>[4x]GPGNEVTLLDSRSVQGELGWIASPLEGGWEEVSIMDEKNTPIRTYQVCNVMEPSQNNWLRTDWITREGAQRVYIEIKFTLRDCNSLPGVMGTCKETFNLYYYESDNDKERFIRENQFVKID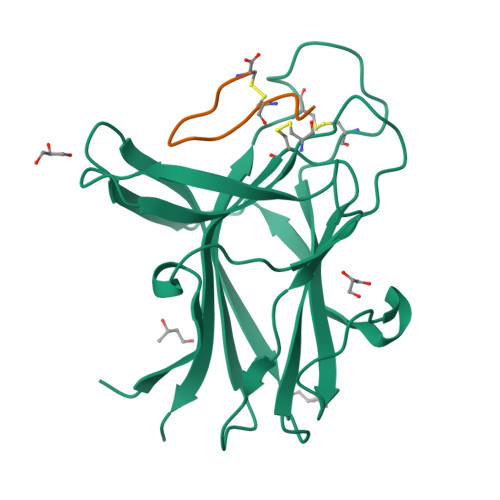TIAADESFTQVDIGDRIMKLNTEIRDVGPLSKKGFYLAFQDVGACIALVSVRVFYKKA;>APYCVYRGSWSC[4x]> MRSKHLVTLFIITFLSFSTVKVWGKDVFAGFVTKKLKTLLDCNFALYYNFKGNGPDAGSFLDFVDEPEQFYWFVEHFLSVKFRVPKHLKDKNIHNFTPCLNRSWVSEFLKEYEEPFVNPVMKFLDKEQRLFFTYNFGDVEPQGKYTYFPVKEFHKYCILPPLIKTNIKDGESGEFLKYQLNKEEYKVFLSSVGSQMTAIKNLYSTVEDEQRKQLLKVIIENESTNDISVQCPTYNIKLHYTKECANSNNILKCIDEFLRKTCEKKTESKHPSADLCEHLQFLFESLKNPYLDNFKKFMTNSDFTLIKPQSVWNVPIFDIYKPKNYLDSVQNLDTECFKKLNSKNLIFLSFHDDIPNNPYYNVELQEIVKLSTYTYSIFDKLYNFFFVFKKSGAPISPVSVKELSHNITDFSFKEDNSEIQCQNVRKSLDLEVDVETMKGIAAEKLCKIIEKFILTKDDASKPEKSDIHRGFRILCILISTHVEAYNIVRQLLNMESMISLTRYTSLYIHKFFKSVTLLKGNFLYKNNKAIRYSRACSKASLHVPSVLYRRNIYIPETFLSLYLGLSNLVSSNPSSPFFEYAIIEFLVTYYNKGSEKFVLYFISIISVLYINEYYYEQLSCFYPKEFELIKSRMIHPNIVDRILKGIDNLMKSTRYDKMRTMYLDFESSDIFSREKVFTALYNFDSFIKTNEQLKKKNLEEISEIPVQLETSNDGIGYRKQDVLYETDKPQTMDEASYEETVDEDAHHVNEKQHSAHFLDAIAEKDILEEKTKDQDLEIELYKYMGPLKEQSKSTSAASTSDEIS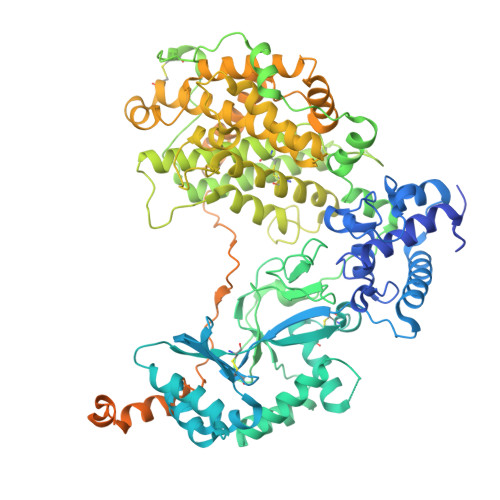GSEGPSTESTSTGNQGEDKTTDNTYKEMEELEEAEGTSNLKKGLEFYKSSLKLDQLDKEKPKKKKSKRKKKRDSSSDRILLEESKTFTSENEL{(1S,2R)-2-[4-(1H-tetrazol-5-yl)benzene-1-carbonyl]cyclopentyl}acetic acid | 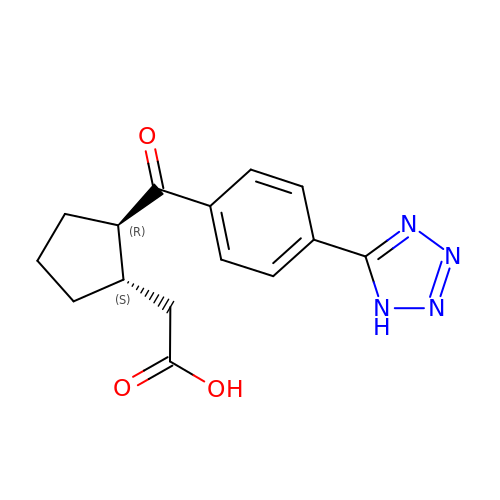C15 H16 N4 O3 | IOEUDWHXQXYIDQ-NWDGAFQWSA-N> GYIQERLKSLND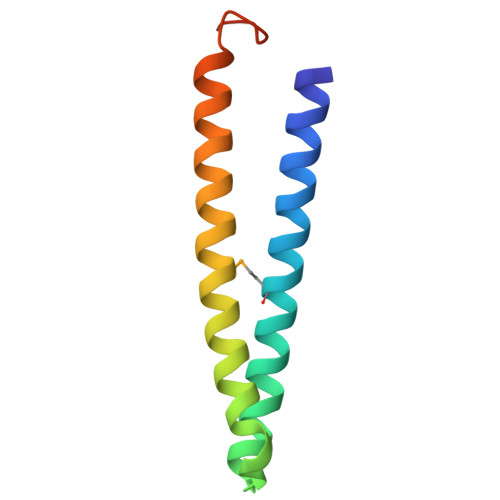IETQLCSMLQEASQVTFIFGELKRGNESVKPQFENHVKQFYERLDKSTTQLRKEIQLLDENVGTRLLPINVNKK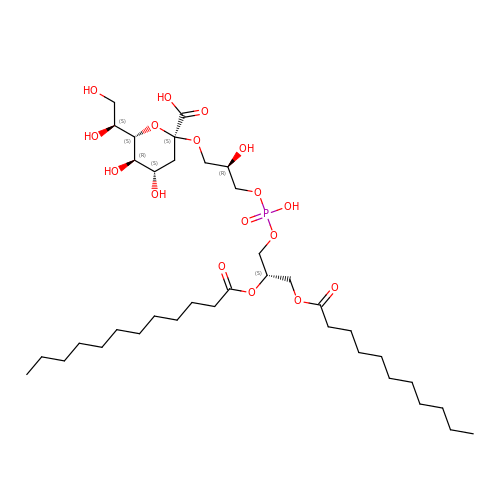(2R,5S,8S)-2,5-dihydroxy-5,10-dioxo-8-[(undecanoyloxy)methyl]-4,6,9-trioxa-5lambda~5~-phosphahenicosan-1-yl 3-deoxy-alpha-L-altro-oct-2-ulopyranosidonic acid | C37 H69 O17 P | ATJBCTLIIQRQQQ-KWTBEUQISA-N>[2x]GSAMDSSRRQYQEKYKQVEQYMSFHKLPADFRQKIHDYYEHRYQGKMF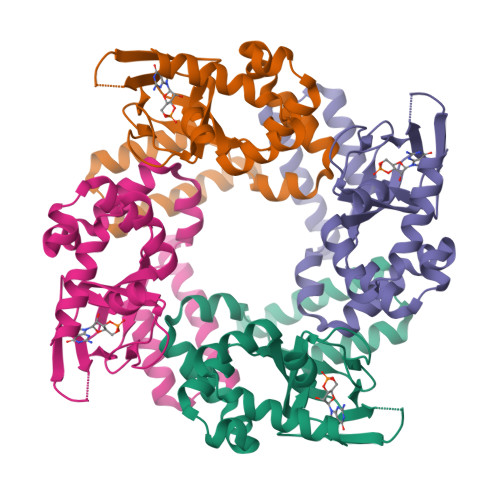DEDSILGELNGPLREEIVNFNCRKLVASMPLFANADPNFVTAMLTKLKFEVFQPGDYIIREGTIGKKMYFIQHGVVSVLTKGNKEMKLSDGSYFGEICLLTRGRRTASVRADTYCRLYSLSVDNFNEVLEEYPMMRRAFETVAIDRLDRIGKKNSILLH> ADEIGDAAKKLGDASYAFAKEVDWNNGIFLQAPGKLQPLEALKAIDKMIVMGAAADPKLLKAAAEAHHKAIGSVSGPNGVTSRADWDSVNAALGRVIASVPENMVMDVYDSVSKITDPKVPAYMKSLVNGADAEKAYEGFLAFKDVVKKS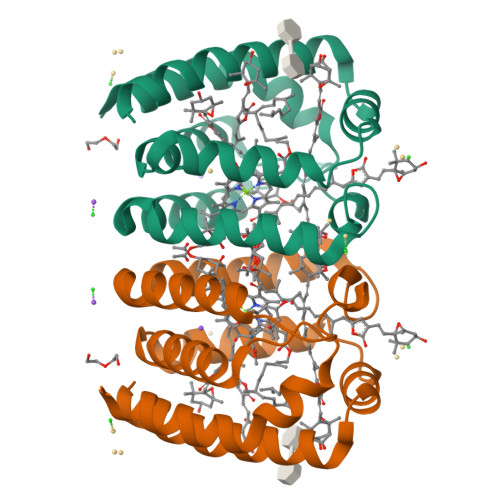Q>[2x]MGAGKFVVGGNWKCNGTLASIETLTKGVAASVDAELAKKVEVIVGVPFIYIPKVQQILAGEANGANILVSAENAWTKSGAYTGEVHVGMLVDCQVPYVILGHSERRQIFHESNEQVAEKVKVAIDAGLKVIACIGETEAQRIANQTEEVVAA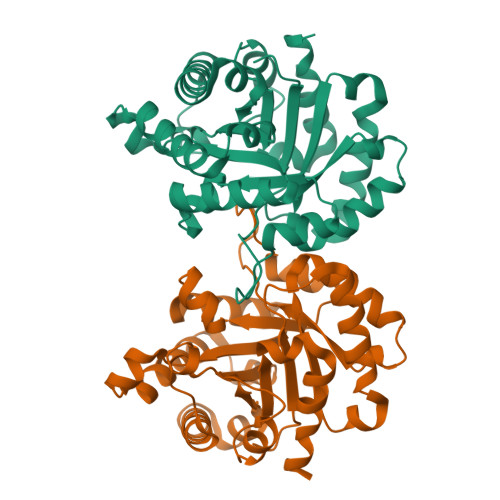QLKAINNAISKEAWKNIILAYEPVWAIGTGKTATPDQAQEVHQYIRKWMTENISKEVAEATRIQYGGSVNPANCNELAKKADIDGFLVGGASLDAAKFKTIINSVSEKL>[2x]MDALSNGIKKHRTSLPSPMFSRNDFSIWSILRKCIGMELSKITMPVIFNEPLSFLQRLTEYMEHTYLIHKASSLSDPVERMQCVAAFAVSAVASQWERTGKPFNPLLGETYELVRDDLGFRLISEQVSHHPPISAFHAEGLNNDFIFHGSIYPKLKFWGKSVEAEPKGTITLELLEHNEAYTWTNPTCCVHNIIVGKLW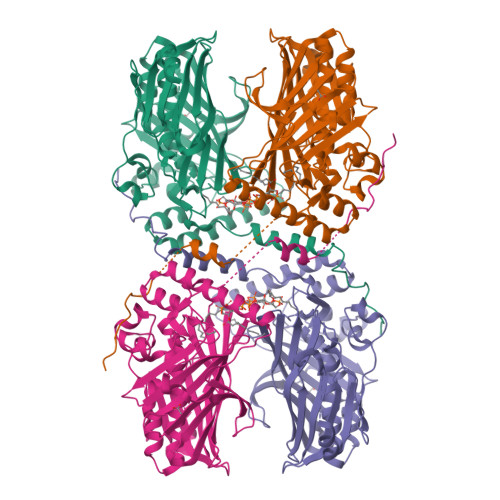IEQYGNVEIINHKTGDKCVLNFKPCGLFGKELHKVEGYIQDKSKKKLCALYGKWTECLYSVDPATFDAYKKNDKKNTEEKKNSKQMSTSEELDEMPVPDSESVFIIPGSVLLWRIAPRPPNSAQMYNFTSFAMVLNEVDKDMESVIPKTDCRLRPDIRAMENGEIDQASEEKKRLEEKQRAARKNRSKSEEDWKTRWFHQGPNPYNGAQDWIYSGSYWDRNYFNLPDIYLEHHHHHH(8alpha,10alpha,13alpha)-6-methylideneandrosta-1,4-diene-3,17-dione | C20 H24 O2 | 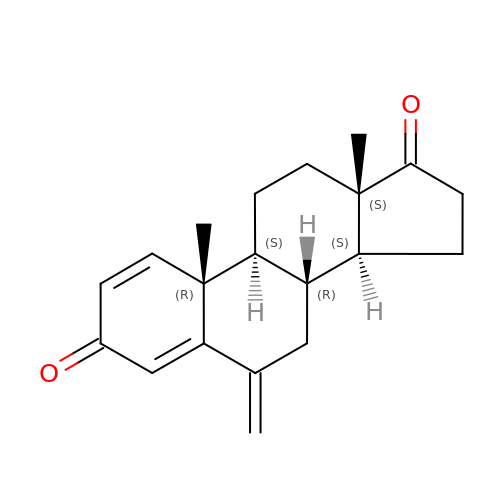BFYIZQONLCFLEV-DAELLWKTSA-N>[2x]MSTVESALTRRIMGIETEYGLTFVDGDSKKLRPDEIARRMFRPIVEKYSSSNIFIPNGSRLYLDVGSHPEYATAECDNLTQLINFEKAGDVIADRMAVDAEESLAKEDIAGQVYLFKNNVDSVGNSYGCHENYLVGRSMPLKALGKRLMPFLITRQLICGAGRIHHPNPLDKGESFPLGYCISQRSDHVWEGVS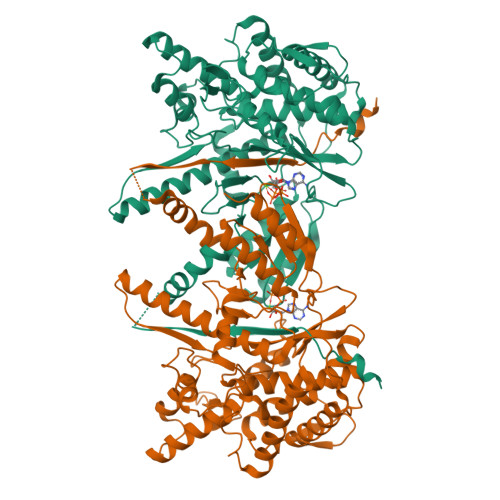SATTRSRPIINTRDEPHADSHSYRRLHVIVGDANMAEPSIALKVGSTLLVLEMIEADFGLPSLELANDIASIREISRDATGSTLLSLKDGTTMTALQIQQVVFEHASKWLEQRPEPEFSGTSNTEMARVLDLWGRMLKAIESGDFSEVDTEIDWVIKKKLIDRFIQRGNLGLDDPKLAQVDLTYHDIRPGRGLFSVLQSRGMIKRWTTDEAILAAVDTAPDTTRAHLRGRILKAADTLGVPVTVDWMRHKVNRPEPQSVELGDPFSAVNSEVDQLIEYMTVHAESYRSKSSVEHHHHHH Merkel cell polyomavirus (MCPyV) is a human double-stranded DNA tumor virus. MCPyV cell entry is unique among members of the polyomavirus family as it requires the engagement of two types of glycans, sialylated oligosaccharides and sulfated glycosaminoglycans (GAGs). On the virus side, PyV-receptor interactions are mediated entirely by the major capsid protein VP1, which forms the capsid outer layer. VP1 assembles into 72 pentameric capsomers, giving rise to small capsids of 45 to 50 nm in diameter.

Using the fVLP preparation, we solved crystallographic and cryo-EM structures of the outer (VP1-only) MCPyV capsid. The structures have 3.5-Å and 3.4-Å resolutions, with no significant differences between them. Overall, six VP1 conformations can be distinguished within the capsid, five from a local capsomer and one from a neighboring strict capsomer, previously annotated with the Greek letters α′, α″, β, β′, γ, and α, respectively. This asymmetric unit of six VP1 chains is sufficient to reconstruct the whole capsid by applying 60-fold icosahedral symmetry. In MCPyV, we observed clear density for five out of potentially six disulfide bridges that connect individual VP1 chains within the strict and local pentamers, respectively, i.e., for the α-α, α′-α″, α″-β, β-β′, and γ-α′ linkages. The MCPyV cryo-EM data further support the presence of this intrapentameric disulfide bond pattern; nonetheless, only the α-α connection is clearly visible in the electrostatic potential map. On the other hand, the MCPyV VP1 sequence harbors a 37-amino-acid (aa) C-terminal extension with unknown function and no detectable homology. Neither in the crystallographic electron density nor in the cryo-EM map was this extension visible. Instead, the most-C-terminal residue resolved in either map is Val388γ (from the so-called γ-chain [see below for an explanation of the chain annotation]), meaning that a stretch of 35 amino acids is completely invisible and thus most likely flexible. However, it is clear from the electron density and electron potential maps that the missing extension must be located on the exterior of the capsid.

>MAPKRKASSTCKTPKRQCIPKPGCCPNVASVPKLLVKGGVEVLSVVTGEDSITQIELYLNPRMGVNSPDLPTTSNWYTYTYDLQPKGSSPDQPIKENLPAYSVARVSLPMLNEDITCDTLQMWEAISVKTEVVGISSLINVHYWDMKRVHDYGAGIPVSGVNYHMFAIGGEPLDLQGLVLDYQTQYPKTTNGGPITIETVLGRKMTPKNQGLDPQAKAKLDKDGNYPIEVWCPDPSKNENSRYYGSIQTGSQTPTVLQFSNTLTTVLLDENGVGPLCKGDGLFISCADIVGFLFKTSGKMALHGLPRYFNVTLRKRWVKNPYPVVNLINSLFSNLMPKVSGQPMEGKDNQVEEVRIYEGSEQLPGDPDIVRFLDKFGQEKTVYPKPSVAPAAVTFQSNQQDKGKAPLKGPQKASQKESQTQEL[6x]>MGSSHHHHHHSSGPQQGLRSNSDDAEKPVVPVPTGDVAIYTTTSSLTRDLTRDAVNFSPKDNLAPTTITLNPAEQYQTMDGFGAAITGSTCYNLLLMKPADRHAFLTETFSDKDGFGFSYIRISIGCSDFSLSEYTCCDTKGIENFALQSEEKDYILPILKEILAINPSIKVIAAPWTCPKWMKVKSLTDRTPLDSWTNGQLNPDYYQDYATYFVKWIQAFKAEGIDIYAVTPQNEPLNRGNSASLYMEWEEQRDFVKTALGPQMKAAGLSTKIYAFDHNYNYDNIESQKNYPGKIYEDAAASQYLAGAAYHNYGGNREELLNIHQAYPEKELLFTETSIGTWNSGRDLSKRLMEDMEEVALGTINNWCKGVIVWNLMLDNDRGPNREGGCQTCYGAVDINNSDYKTIIRNSHYYIIAHLSSVVKPGAVRIATTGYTDNGITCSAFENTDGTYAFVLINNNEKSKKITVSDGQRHFAYDVPGKSVTSYRWAKSK[3x]

Our data show that this locus orchestrates the degradation of 1,6-β-glucan, and this enables B. thetaiotaomicron to utilize this fungal polysaccharide. The critical enzyme encoded by the PUL is BT3312, an endo-1,6-β-glucanase that is displayed on the bacterial surface, allowing direct access to the intact glycan. The enzyme showed no activity on 1,3-β-glucan, 1,4-β-glucan, or 1,6-β-galactan but was active on the 1,6-β-glucan pustulan, producing a range of oligosaccharides in the initial phases of the degradative process. The crystal structure of the endo-1,6-β-glucanase shows that substrate recognition is mediated by shape complementarity of the substrate-binding cleft and the hooked U-shaped conformation of 1,6-β-glucan, rather than through extensive hydrogen-bonding interactions with the polysaccharide.

Thus, to explore the mechanism of catalysis and substrate binding of an endo-1,6-β-glucanase, the crystal structure of BT3312 was determined in complex with the ligand β-glucosyl-1,6-deoxynojirimycin (GlcDNJ). In the ligand complex, unambiguous electron density corresponding to GlcDNJ was evident. The structure of BT3312 bound to GlcDNJ reveals details of the active site and the distal substrate-binding subsites. The Glc at the −2 subsite adopts a relaxed chair (4C1) conformation, whereas DNJ bound in the −1 subsite, the active site, is distorted and adopts a 4E envelope conformation. Within the −1 subsite, the carboxylate of Glu339 and Nδ2 of Asn237 make polar contacts with O2. Binding of GlcDNJ in the active site is also mediated through apolar contacts between the sugar ring and Trp377, which provides the hydrophobic platform in the −1 subsite. The catalytic nucleophile, Glu339, is 3.2 Å from the anomeric carbon of DNJ and is thus in an appropriate position to mount a nucleophilic attack on the anomeric carbon. Glu238 is in an optimal position (3.4 Å) to donate a proton to the glycosidic oxygen appended to C1 and thus is able to function as the acid-base catalyst. The −2 subsite makes only apolar interactions with the Glc in GlcDNJ. Trp345 stacks against the pyranose ring, whereas the disulfide formed by Cys393 and Cys396 also makes apolar contacts with the −2 Glc.> MAYDGLFTKKMVESLQFLTTGRVHKINQPDNDTILMVVRQNRQNHQLLLSIHPNFSRLQLTTKKYDNPFNPPMFARVFRKHLEGGIIESIKQIGNDRRIEIDIKSKDEIGDTIYRTVILEIMGKHSNLILVDENRKIIEGFKHLTPNTNHYRTVMPGFNYEAPPTQHKINPYDITGAEVLKYIDFNAGNIAKQLLNQFEGFSPLITNEIVSRRQFMTSSTLPEAFDEVMAETKLPPTPIFHKNHETGKEDFYFI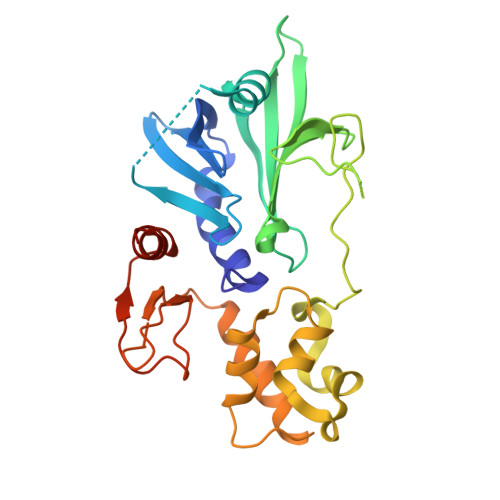KLNQFNDDTVTYDSLNDLLDRFYDARGERERVKQ>[4x]MVSVINTVDTSHEDMIHDAQMDYYGTRLATCSSDRSVKIFDVRNGGQILIADLRGHEGPVWQVAWAHPMYGNILASCSYDRKVIIWREENGTWEKSHEHAGHDSSVNSVCWAPHDYGLILACGSSDGAISLLTYTGEGQWEVKKINNAHTIGCNAVSWAPAVVPGSLIDHPSGQKPNYIKRFASGGCDNLIKLWKEEEDGQWKEEQKLEAHSDWVRDVAWAPSIGLPTSTIASCSQDGRVFIWTCDDASSNTWSPKLLHKFNDVVWHVSWSITANILAVSGGDNKVTLWKESVDGQWVCISDVNKGQGSVSASVTE;>[4x]MGSSHHHHHHSGDPFSECNDEIDNAKLIMKERRFTASYTFAKFSTGSMLLTKDIVGKSGVSIKRLPTELQRKFLFDDVYLDKEIEKVTIEA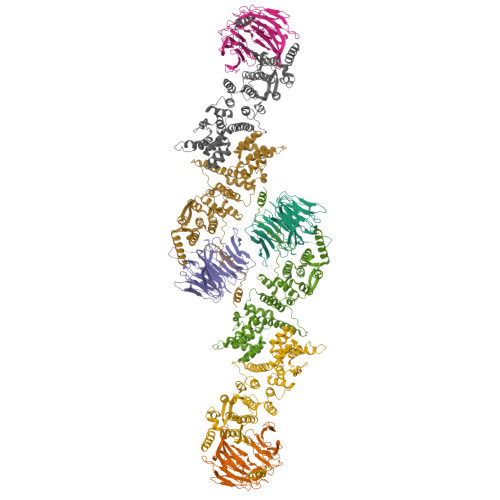RKSNPYPQISESSLLFKDALDYMEKTSSDYNLWKLSSILFDPVSYPYKTDNDQVKMALLKKERHCRLTSWIVSQIGPEIEEKIRNSSNEIEQIFLYLLLNDVVRASKLAIESKNGHLSVLISYLGSNDPRIRDLAELQLQKWSTGGCSIDKNISKIYKLLSGSPFEGLFSLKELESEFSWLCLLNLTLCYGQIDEYSLESLVQSHLDKFSLPYDDPIGVIFQLYAANENTEKLYKEVRQRTNALDVQFCWYLIQTLRFNGTRVFSKETSDEATFAFAAQLEFAQLHGHSLFVSCFLNDDKAAEDTIKRLVMREITLLRASTNDHILNRLKIPSQLIFNAQALKDRYEGNYL> AHHHHHHGSKLKFWREVAIDIISDFETTIMPFFGNPDGGKLVKISPSGDETKLVDKLAEDLILSRITELGVNVVSEEVGVIDNESEYTVIVDPLDGSYNFIAGIPFFALSLAVFKKDKPIYAIIYEPMTERFFEGIPGEGAFLNG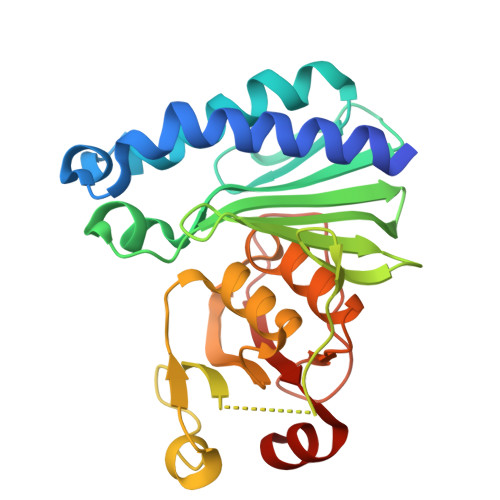KRIKVRKTPDEKPSISFYSRGKGHEIVKHVKRTRTLGAIALELAYLAMGALDGVVDVRKYVRPTDIAAGTIIAKEAGALIKDSAGKDIDISFNATDRLDVIAVNSEELLKTILSLLE> MGNYKKPKLLYCSNGGHFLRILPDGTVDGTRDRSDQHIQLQLSAESVGEVYIKSTETGQYLAMD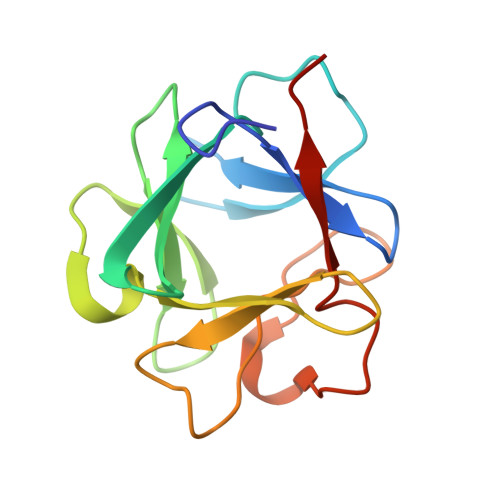TDGLLYGSQTPNEECLFLERLEENHYNTYISKKHAEKNWFVGLKKNGSCKRGPRTHYGQKAILFLPLPVSSD> TTLLNPYFGEFGGMYVPQILMPALNQLEEAFVSAQKDPEFQAQFADLLKNYAGRPTALTKCQNITAGTRTTLYLKREDLLHGGAHKTNQVLGQALLAKRMGKSEIIAETGAGQHGVASALASALLGLKCRIYMGAKDVERQSPNVFRMRLMGAEVIPVHSGSATLKDLWNEALRDWSGSYETAHYMLGTAAGPHPYPTIVREFQRMIGEETKAQILDKEGRLPDAVIACVGGGSNAIGMFADFINDTSVGLIGVEPGGHGIETGEHGAPLKHGRVGIYFGMKAPMMQTADGQIEESYSISAGLDFPSVGPQHAYLNSIGRADYVSITDDEALEAFKTLCRHEGIIPALESSHALAHALKMMREQPEKEQLLVVNLSGRGDKD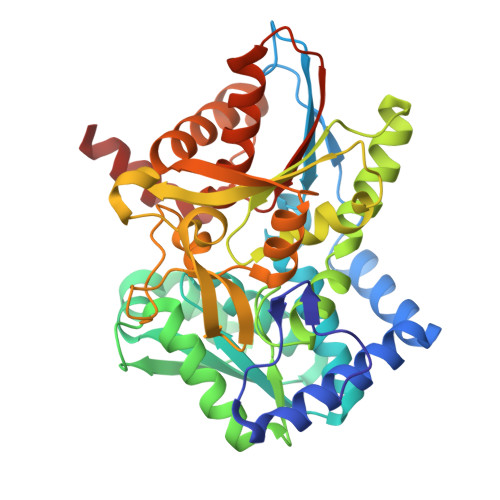IFTVHDILKARGEI> GAGCAGACCAGACGCCACTCA;> CGTCT;> 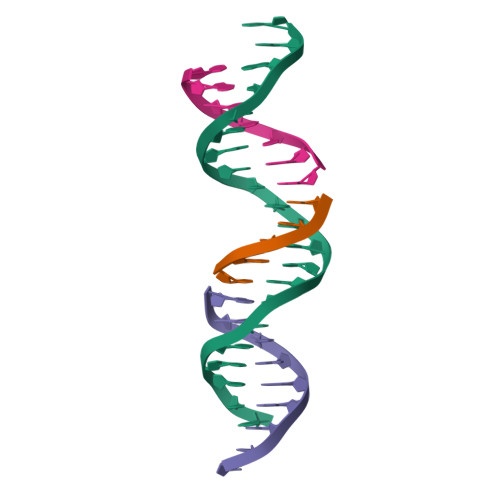TCTGAGTGG;> GGTCTGC> MSLDYDLLIKNGQTVNGMPVEIAIKEKKIAAVAATISGSAKETIHLEPGTYVSAGWIDDHVHCFEKMALYYDYPDEIGVKKGVTTVIDAGTTGAENIHEFYDLAQQAKTNVFGLVNISKWGIVAQDELADLSKVQASLVKKAIQELPD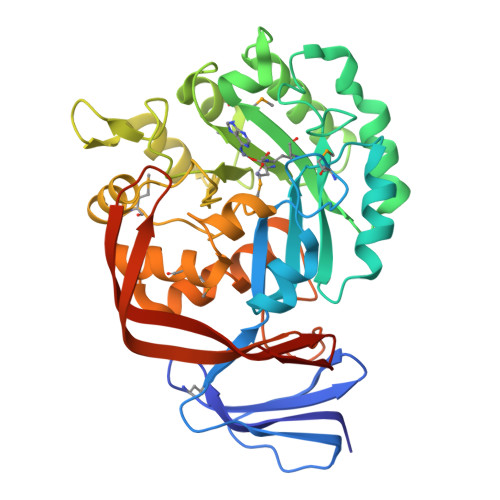FVVGIKARMSRTVIGDNGITPLELAKQIQQENQEIPLMVHIGSAPPHLDEILALMEKGDVLTHCFNGKENGILDQATDKIKDFAWQAYNKGVVFDIGHGTDSFNFHVAETALREGMKAASISTDIYIRNRENGPVYDLATTMEKLRVVGYDWPEIIEKVTKAPAENFHLTQKGTLEIGKDADLTIFTIQAEEKTLTDSNGLTRVAKEQIRPIKTIIGGQIYDNEGHHHHHH>[2x]LILNLRGGAFVSNTQITMADKQKKFINEIQEGDLVRSYSITDETFQQNAVTSIVKHEADQLCQINFGKQHVVCTVNHRFYDPESKLWKSVCPHPGSGISFLKKYDYLLSEEGEKLQITEIKTFTTKQPVFIYHIQVENNHNFFANGVLAHAMQVSI;>[2x]LILNLRGGAFVSNTQIT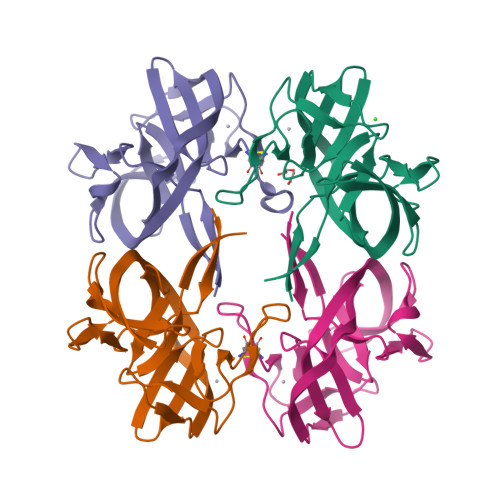MADKQKKFINEIQEGDLVRSYSITDETFQQNAVTSIVKHEADQLCQINFGKQHVVCTVNHRFYDPESKLWKSVCPHPGSGISFLKKYDYLLSEEGEKLQITEIKTFTTKQPVFIYHIQVENNHNFFANGVLAHAMQVS>[2x]MGSSHHHHHHSQDPAEKQKHDGRVKIGHYVLGDTLGVGTFGKVKIGEHQLTGHKVAVKILNRQKIRSLDVVGKIKREIQNLKLFRHPHIIKLYQVISTPTDFFMVMEYVSGGELFDYICKHGRVEEMEARRLFQQILSAVDYCHRHMVVHRDLKPENVLLDAHMNAKIADFGLSNMMSDGEFLRTSCGSPNYAAPEVISGRLYAGPEVDIWSCGVILYALLCGTLPFDDEHVPTLFKKIRGGVFYIPEYLNRSVATLLMHMLQVDPLKRATIKDIREHEWFKQGLPSYLFPEDPSYDANVIDDEAVKEVCEKFECTESEVMNSLYSGDPQDQLAVAYHLIIDNRRIMNQASEFYLASSPPSGSFMDDSAMHIPPGLKPHPERMPPLIADSPKARCPLDALNTTKPKSLAVKKAKWHLGIRSQSKPYDIMAEVYRAMKQLDFEWKVVNAYHLRVRRKNPVTGNYVKMSLQLYLVDNRSYLLDFKSIDDEVVEQRSGSSTPQRSCSAAGLHRPRSSFDSTTAESHSLSGSLTGSLTGSTLSSVSPRLGSHTMDFFEMCASLITTLAR;>MGNTSSERAALERHGGHKTPRRDSSGGTKDGDRPKILMDSPEDADLFHSEEIKAPEKEEFLAWQHDLEVNDKAPAQARPTVFRWTGGGKEVYLSGSFNNWSKLPLTRSHNNFVAILDLPEGEHQYKFFVDGQWTHDPSEPIVTSQLGTVNNIIQVKKTDFEVFDALMVDSQKCSDVSELSSSPPGPYHQEPYVCKPEERFRAPPILPPHLLQVILNKDTGISCDPALLPEPNHVMLNHLYALSIKDGVMVLSATHRYKKKYVTTLLYKPI[2x];>[2x]MADLNWETVISSDSSPAVENEHPQETPESNNSVYTSFMKSHRCYD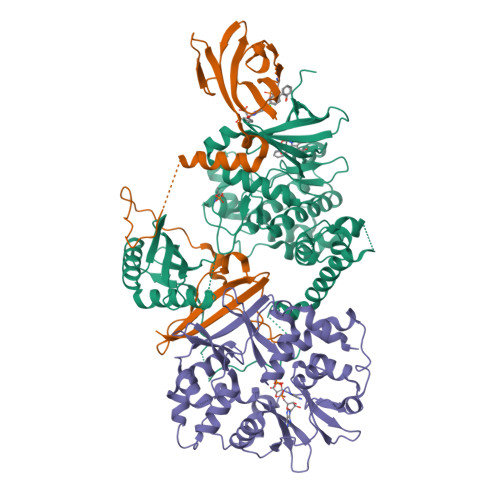LIPTSSKLVVFDTSLQVKKAFFALVTNGVRAAPLWDSKKQSFVGMLTITDFINILHRYYKSALVQIYELEEHKIETWREVYLQDSFKPLVCISPNASLFDAVSSLIRNKIHRLPVIDPESGNTLYILTHKRILKFLKLFITEFPKPEFMSKSLEELQIGTYANIAMVRTTTPVYVALGIFVQHRVSALPVVDEKGRVVDIYSKFDVINLAAEKTYNNLDVSVTKALQHRSHYFEGVLKCYLHETLETIINRLVEAEVHRLVVVDENDVVKGIVSLSDILQALVLTGGEKKP>YEHTAVMPNKVGIPYKALVERPGYAPVHLQIQLVNTRIIPSTNLEYITCKYKTKVPSPVVKCCGATQCTSKPHPDYQCQVFTGVYPFMWGGAYCFCDTENTQMSEAYVERSEECSIDHAKAYKVHTGTVQAMVNITYGSVSWRSADVYVNGETPAKIGDAKLIIGPLSSAWSPFDNKVVVYGHEVYNYDFPEYGTGKAGSFGDLQSRTSTSNDLYANTNLKLQRPQAGIVHTPFTQAPSGFERWKRDKGAPLNDVAPFGCSIALEPLRAENCAVGSIPISIDIPDAAFTRISETPTVSDLECKITECTYASDFGGIATVAYKSSKAGNCPIHSPSGVAVIKENDVTLAESGSFTFHFSTANIHPAFKLQVCTSAVTCKGDCKPPKDHIVDYPAQHTESFTSAISATAWSWLKVLVGGTSAFIVLGLIATAVVALVLFFHRH[6x];>[6x]DLDTHFTQYKLARPYIADCPNCGHSRCDSPIAIEEVRGDAHAGVIRIQTSAMFGLKTDGVDLAYMSFMNGKTQKSIKIDNLHVRTSAPCSLVSHHGYYILAQCPPGDTVTVGFHDGPNRHTCTVAHKVEFRPVGREKYRHPPEHGVELPCNRYTHKRADQGHYVEMHQPGLVADHSLLSIHSAKVKITVPSGAQVKYYCKCPDVREGITSSDHTTTCTDVKQCRAYLIDNKKWVYNSGRLPRGEGDTFKGKLHVPFVPVKAKCIATLAPEPLVEHKHRTLILHLHPDHPTLLTTRSLGSDANPTRQWIERPTTVNFTVTGEGLEYTWGNHPPKRVWAQESGEGNPHGWPHEVVVYYYNRYPLTT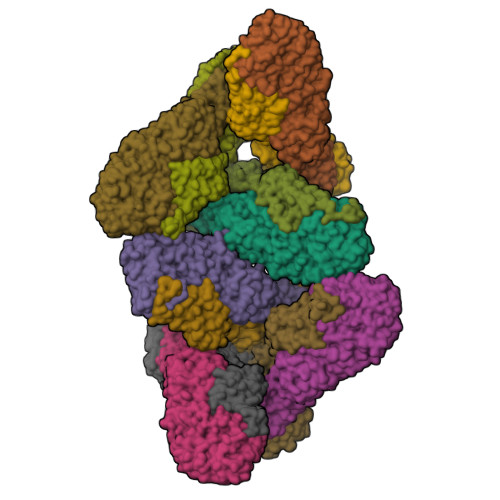IIGLCTCVAIIMVSCVTSVWLLCRTRNLCITPYKLAPNAQVPILLALLCCIKPTRA> MSTPARRRLMRDFKRMKEDAPPGVSASPLPDNVMVWNAMIIGLADTPYEDGTFRLLLEFDEEYPNKPPHVKFLSEMFHPNVYANGEICLDILQNRWTPTYDVASILTSIQSLFNDPNPASPANVEAATLFKDHKSQYVKRVKETVEKSWE;>MTAEPATKKIKLELSDPSEPLTQSDVIAFQKEALFRCINRRRVDFEALRKQYELSRRECIDVSRKLANIMALIVTLARFIETFCTDANEKQLCREIAQGDETLIVQRSDSFMKLLTKYGKPNTTDSNT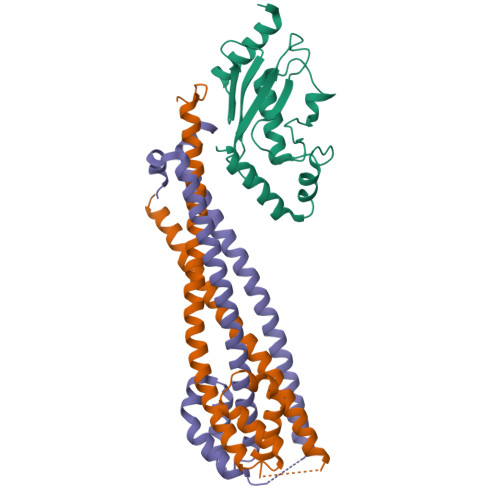NSNASDHIQELTTELKNLRKSKEELFYENSQLTEEISALKEYYTNIIRKYDRDESFTIKRVFKEDKTDAVKELREDEKESNENN[2x]> KYIPRIAEDMTIQEAKKFARENNIKEGKIDEIMHDSIQDTAEQKVQLLLCWYQSH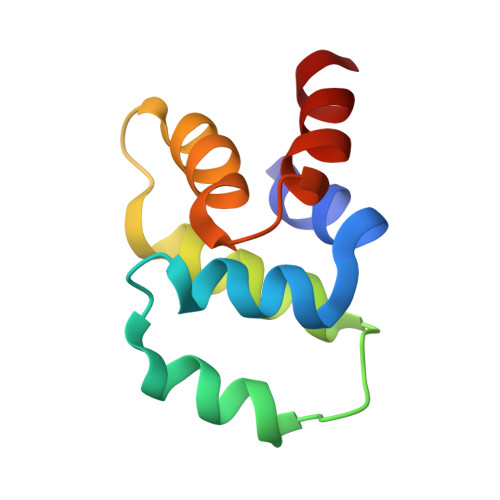GKSDAYQDLIKGLKKAECRRTLDKFQDMVQK[(R)-(2,3-dihydro-1-benzofuran-5-yl){[6-(4-methylphenyl)thieno[2,3-d]pyrimidin-4-yl]amino}methyl]phosphonic 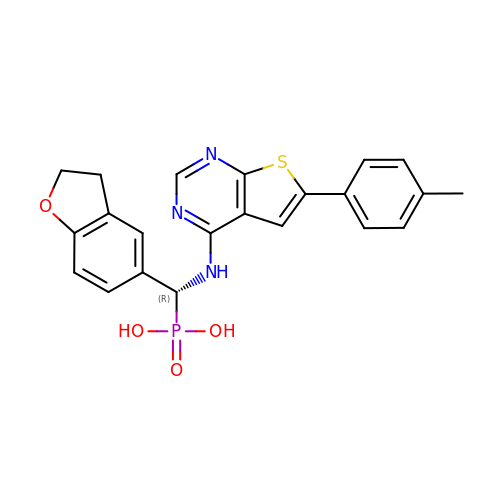acid | C22 H20 N3 O4 P S | ORNKDTLGUAHCGN-OAQYLSRUSA-N> MDEYSELSGIVDPRVLVTTSRDPSSRLMAFSKEIRLMFPTAIRLNRGNLILPDLVMSAQRERLSDIILLHEHRGTPTAITISHFPHGPTLMASLHNVVLRADIPKSIKGTVSESYPHLIFEGFRTPLGQRVVKILKHLFPPRDPTNNAKSGNRVITFVNQDDCI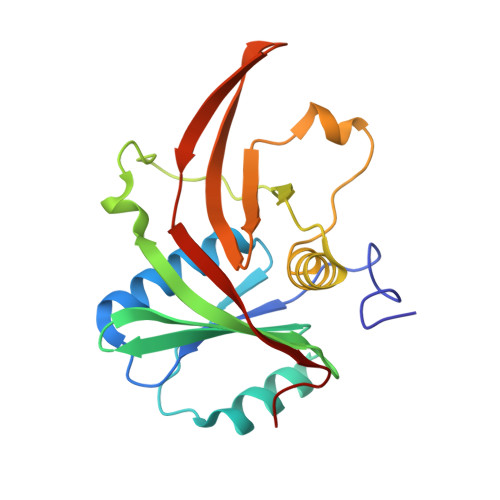EVRHHVYVRTNYNSVELSEVGPRFTMRPFSITMGTLE> GEDPSLDRPFISEGTTLKDLIYDMTTSGSGSGLPLLVQRTIARTIVLQESIGKGRFGEVWRGKWRGEEVAVKIFSSREERSWFREAEIYQTVMLRHENILGFIAADNKDNGTWTQLWLVSDYHEHGSLFDYLNRYTVTVEGMIKLALSTASGLAHLHMEIVGTQGKPAIAHRDLKSKNILVKKNGTCCIADLGLAVRHDSATDTIDIAPNHRVGTKRYMAPEVLDDSINMKHFESFKRADIYAMGLVFWEIARRCSIGGIHEDYQ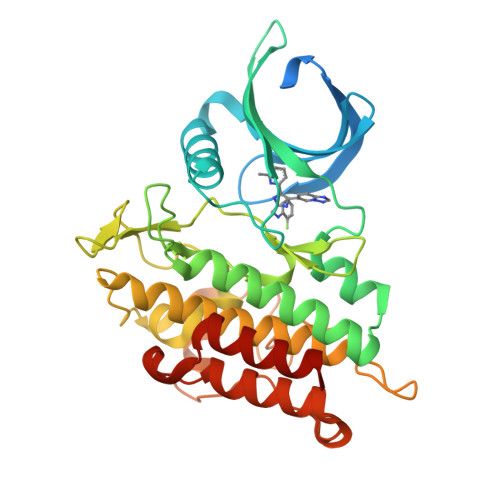LPYYDLVPSDPSVEEMRKVVCEQKLRPNIPNRWQSCEALRVMAKIMRECWYANGAARLTALRIKKTLSQLSQQEGIKM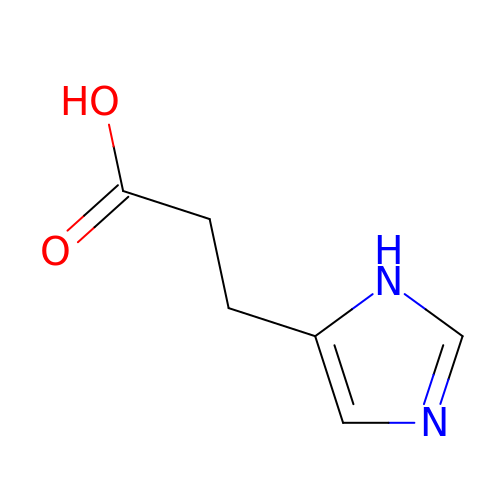3-(1~{H}-imidazol-5-yl)propanoic acid | C6 H8 N2 O2 | ZCKYOWGFRHAZIQ-UHFFFAOYSA-N> AANEADYQAKLTAYQTELARVQKANADAKAAYEAAVAANNAANAALTAENTAIKKRNADAKADYEAKLAKYQADLAKYQKDLADYPVKLKAYEDEQTSIKAALAELEKHKNEDGNLTEPSAQNLVYDLEPNANLSLTTDGKFLKASAVDDAFSKSTSKAKYDQKILQLDDLDITNLEQSNDVASSMELYGNFGDKAGWSTTVSNNSQVKWGSVLLERGQSATATY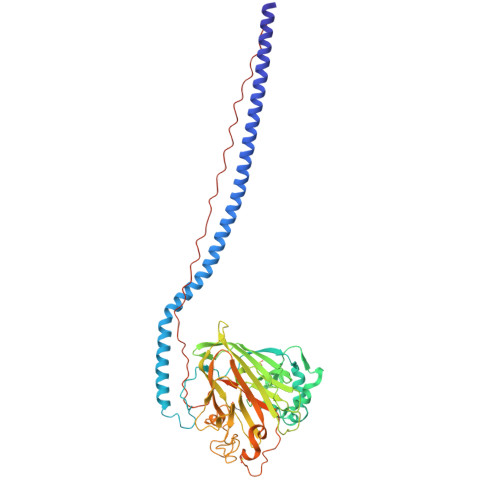TNLQNSYYNGKKISKIVYKYTVDPKSKFQGQKVWLGIFTDPTLGVFASAYTGQVEKNTSIFIKNEFTFYDEDGKPINFDNALLSVASLNREHNSIEMAKDYSGKFVKISGSSIGEKNGMIYATDTLNFKQGEGGSRWTMYKNSQAGSGWDSSDAPNSWYGAGAIKMSGPNNYVTVGATSATNVMPVSDMPVVPGKDNTDGKKPNIWYSLNGKIRAVNVPKVTKEKPTPPVKPTAPTKPTYETEKPLKPAPVAPNYEKEPTPPTRLEHHHHHH The exocyst is an evolutionarily conserved octameric protein complex that mediates the tethering of post-Golgi secretory vesicles to the plasma membrane. Most syntaxin proteins contain an N-terminal region that autonomously folds into a three-helix bundle (the ‘Habc domain') that interacts intramolecularly with their SNARE motif to generate a ‘closed' conformation, which, in many cases, blocks its assembly into the SNARE complex345678910. The rate-limiting step is the interaction between Sso and Sec9, which is hindered by the auto-inhibition of Sso. Here we report that the exocyst subunit Sec3 directly interacts with Sso1/2, and promotes the initial assembly of the Sso-Sec9 t-SNARE complex and stimulates membrane fusion.

We have obtained the crystal structure of the Sec3–Sso2 complex under two different crystallization conditions, both of which demonstrate that the binding of Sec3 leads to conformational changes on Sso that is crucial for the relief of its auto-inhibition. Consistent with previously reports of Sec3 lipid-binding domain2324, the core of Sec3N folds into a PH domain that contains a β-barrel formed by two sets of β-sheet with a helix capping one end. The interface between Sec3N and Sso2 is ∼700 Å2, which is mediated primarily by 13 hydrogen bonds and 10 salt bridges. The seven main interface residues on Sec3 consist of K149, Q219, E222, H224, Y237, R241 and R245, which together describe a horseshoe-like shape on a relatively flat surface of the Sec3 PH domain. These residues provide a platform to make extensive contacts with Hc of Sso2, and some contacts with the SNARE motif of Sso2. In the Sso2-Sec3 crystal structure, the N terminus of the H3 domain bends approximately 22° away from its original position, and is tilted towards the Ha domain. The crystal structure suggests that Sec3 interaction causes the bending of the SNARE motif, which then led to the disruption of the hydrophobic interactions in the core of Sso2 involving HL2. Such changes could facilitate the release of the SNARE motif of Sso2 from its Habc domain when Sec9 is available. The four Sec3/Sso2 dimers in the two crystal forms are essentially identical. Both the bending of the SNARE motif N-terminus and the relaxation of HL2 of Sso2 described above are found in all four copies of the Sec3/Sso2 complex present in the two different crystal forms.

>[3x]GSHMDFVAFMNKINSINANLSRYENIINQIDAQHKDLLTQVSEEQEMELRRSLDDYISQATDLQYQLKADIKDAQRDGLHDSNKQAQAENCRQKFLKLIQDYRIIDSNYKEESKEQAKRQYTIIQPEATDEEVEAAINDVNGQQIFSQALLNANRRGEAKTALAEVQARHQELLKLEKTMAELTQLFNDMEELVIELTQLFNDMEELVIE;>QGHMSNFLAEQYERDRKAIINCCFSRPDHKTGEPPNNYITHVRIIEDSKFPSSRPPPDSKLENKKKRLLILSAKPNNAKLIQIHKARENSDGSFQIGRTWQLTELVRVEKDLEISEGFILTMSKKYYWETNSAKERTVFIKSLITLYIQTFEGHVPELVNWDLSLFYLDERSYQRAVITNRPGSVSPIKSPTSNFTTNTTQSVGSVPFSAPTERTRRSETESVNPVSTPASVEYHAGMKSLNKAPYSSNS[3x]>MAYFLDFDERALKEWRKLGSTVREQLKKKLVEVLESPRIEANKLRGMPDCYKIKLRSSGYRLVYQVIDEKVVVFVISVGKAERSEVYSEAVK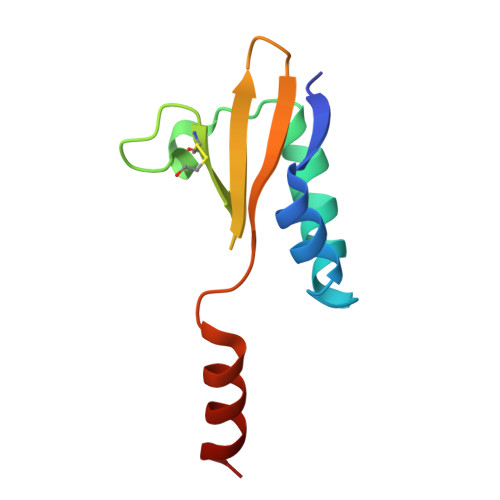RIL[2x]> DFQSESYKDAYSRINAIVIEGEQEAFDNYNRLAEMLPDQRDELHKLAKMEQRHMKGFMACGKNLSVTPDMGFAQKYYERLHENFKAAAAEGKVVTCLLIQSLIIECFAIAAYNIYIPVADAFARKITEGVVRDEYLHRNFGEEWLKANFDASKAELEEANRQNLPLVWLMLNEVADDARELGMERESLVEDFMIAYGEALENIGFTTREIMRMSAYGLAA;> LDFQSESYKDAYSRINAIVIEGEQEAFDNYNRLAEMLPDQRDELHKLAKMEQRHMKGFMACGKNLSVTPDMGFAQKYYERLHENFKAAAAEGKVVTCLLIQSLIIECFAIAAYNIYIPVADAFARKITEGVVRDEYLHRNFGEEWLKANFDASKAELEEANRQNLPLVWLMLNEVADDARELGMERESLVEDFMIAYGEALENIGFTTREIMRMSAYGLAAV

Cyanobacterial aldehyde-deformylating oxygenase (cADO), which catalyzes the conversion of Cn fatty aldehyde to its corresponding Cn-1 alk(a/e)ne, is a key enzyme in that pathway. Cyanobacterial aldehyde-deformylating oxygenase (cADO) belongs to the superfamily of ferritin-like di-iron proteins and contains a di-iron center. To gain insights into the reaction catalyzed by cADO, we determined structures of wild type ADO from Synechococcus elongates PCC7942 (Se) with different treatment (WT0, no treatment; WT1, co-crystallized with iron; WT-HP, soaked in H2O2), and solved the structures of two SeADO mutants (Y122F and F86YF87Y). SeADO belongs to the di-iron protein family, with conserved sequence of two EX28-29EX2H motifs, in which six conservative amino acids from four helices (Glu32 from helix H1, Glu115 from helix H4, Glu60 & His63 from helix H2, and Glu144 & His147 from helix H5) act as metal ligands.

The only exception is molecule B in the F86YF87Y structure, which contains the di-metal cluster while exhibiting the L5 conformation. However, the relatively weak electron density indicates a low occupancy of the two iron atoms in this molecule. In the molecule B of F86YF87Y structure, a segment (from residue 144–150) in helix H5 changes its conformation from helix to loop, which might be induced by the swing of Glu144 observed in WT1 structure. As a consequence, His147 moves away from the active site with a 9Å distance to Fe2. In addition, H63 is located more distantly from the active site, and the ligand bond between Fe1 atom and H63 is broken. The iron ions at the active site are bridged by the residue Glu60 together with a water molecule. The two iron atoms are maintaining their tetrahedral coordinations. The relatively low coordination number in this structure indicates that the active site is in a reduced state, and should be highly sensitive to dioxygen. In addition, a hole is formed at the protein surface as a result of helix H5 distortion, which exposes the di-iron cluster and the bridging water molecule to solvent. We assumed that the hole formed in the F86YF87Y structure serves as the access channel for the co-substrate dioxygen.> MEYTYDVVIIGSGGAGFSAGLEAIAAGRSAVIIEKMPIIGGNSLISGAEMNVAGSWVQKNMGITDSKELFISDTLKGGDFKGDPEMVKTMVDNAVGAAEWLRDYVKVEFYPDQLFQFGGHSVKRALIPKGHTGAEVISKFSIKADEVGLPIHTNTKAEKLIQDQTGRIVGVEAAHNGKTITYHAKRGVVIATGGFSSNMEMRKKYNPELDERYGSTGHAGGTGDGIVMAEKIHAAAKNMGYIQSYPICSPTSGAIALIADSRFFGAVLINQKGERFVEELERRDVISHAILAQPGRYTYVLWNQDIENVAHTVEMHQGELKEFTKDGLMYKVDTLEEAAKVFNIPEDKLLSTIKDVNHYAATGKDEAFNHRSGLVDLSKGPYWILKATPSVHHTMGGLVVDTRTRVLDEQGKVIPGLFAAGEVTGLTHGTNRLGGNAYTDIIVYGRIAGQEAAKHHHHHH

Interestingly, the fecal microbiota of type 2 diabetes patients has an increased capacity to produce imidazole propionate (ImP), which is catalyzed by the bacterial enzyme urocanate reductase (UrdA). The structure of UrdA′ was determined at four specific states: an ADP-bound structure without substrate at 1.1 Å resolution, and three FAD-bound structures in complex with either the substrate urocanate (1.56 Å) or the product ImP (1.40 Å), or without any ligand bound (2.56 Å). The X-ray structure revealed that UrdA′ adopts a two-domain overall structure (FAD domain and clamp domain) connected by a hinge region (identified using the DynDom server). Based on the structural and functional data presented, we suggest that apo-ADP represents an inactive state, while the binding of FAD induces movement of the clamp domain that enables binding of the substrate urocanate to form an active complex with a solvent-accessible channel for water-mediated proton delivery to Arg411, and subsequent protonation of the substrate.

In addition, we obtained a structure of UrdA′ with an ADP instead of FAD. Notably, this structure does not include any bound ligand, even though the sample was supplemented with urocanate (hereafter called apo-ADP). In the apo-ADP structure, an unambiguous density was present for ADP. In addition, density that could be best accommodated by a glycerol molecule was observed in the expected urocanate binding site. The closed conformation of the apo-ADP structure implies that the urocanate cannot be bound when ADP occupies the FAD-binding site, which was supported by the ADP-induced inhibition of UrdA′ activity. When comparing the apo-FAD structure with apo-ADP structure, we also observed that the absence of the flavin group resulted in the clamp domain moving toward the FAD domain, thereby creating a closed, solvent inaccessible conformation. Phe243 is now positioned in the same manner as in the apo-ADP structure.>[12x]MGFKSWITEKLNPGQRIIRDMEPVSHRTNRKPFTTGQAYSKIEILNRTANMVIDSAAECSYTVGDKYNIVTYANGVKTKTLDTLLNVRPNPFMDISTFRRLVVTDLLFEGCAYIYWDGTSLYHVPAALMQVEADANKFIKKFIFNNQINYRVDEIIFIKDNSYVCGTNSQISGQSRVATVIDSLEKRSKMLNFKEKFLDNGTVIGLILETDEILNKKLRERKQEELQLDYNPSTGQSSVLILDGGMKAKPYSQISSFKDLDFKEDIEGFNKSICLAFGVPQVLLDGGNNANIRPNIELFYYMTIIPMLNKLTSSLTFFFGYKITPNTKEVAALTPDKEAEAKHLTSLVNNGII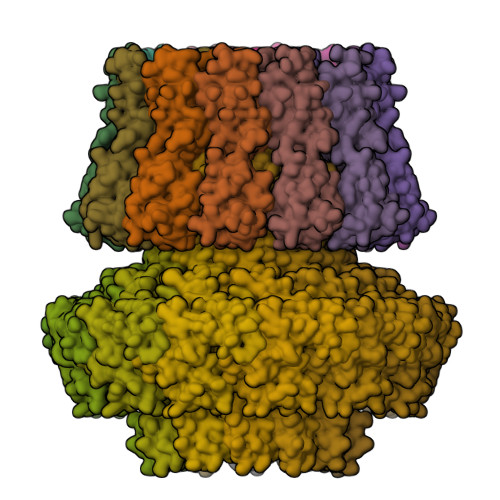TGNEARSELNLEPLDDEQMNKIRIPANVAGSATGVSGQEGGRPKGSTEGD;>MQIITAEDYRLYGGLKRPELESGVEVMITAANALITSLLGMDDADAVDQLITTKPTRKKYFLSSPSATSVTKMTINDKEIDPEQYKLYSDGVILLKFNPPEGYMDVEYTQGGFNPMPEDLKLAACMLVDHWHKQDYRQARTIGGETVTFNNTKSGIPEHIRTIIEVYRRV[12x]> MDIRGRKMKKPPACVQCRKRKIGCDRVKPICGNCMKHNKMDCFYPDVPGQYVPSSSSSSNTRQVANGPYLNSYYASRRVSKETAALLQKNPELASLEQIREYNTRLQLLNAQNQLNNRSSAANATLNQQHTQYIPKSVPSLESKPVTSANESSTPLNWVQGPAIFHMLTSP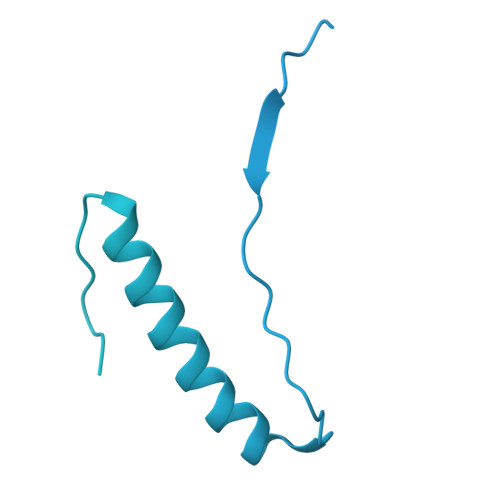YTQDEIINHEMNFLKGRLLELQEITGKKITGVNLDLKQDSSAQMQSSHSNRNQEEFLTIKKRKLSEDGVTDGDGKPIPESERRPHLNEFKDLDPQFLDTNKVFNVFNSAISEEGRNRLWLLPKNINKSSIFQIQYLIERDPFLFKFFNDLNILIETQFNGPLHDLVASRNSIERNSGISQILKFPSQSITQTLINKYLSTITETNSILPILKPKRLLPIVEQLFPSNTINKPNSKDFETIFQVFSVTNDQLLNLGFITLCLLILFESLNSTVLIPLRDDEHLQLFNVLFNYLPLLKSNLTTLRFEIEKRSMCNIETLRFISLWKYYQFVMDTSSSSSFVIDYDEDMHMACLLSLNHETQNQSHILTWNFIFKNYCWRHLFLGQLPLLMSEPFTNSTPIIDPLLNNDFELIDFEVNLMKYLQSKDQQLSIDKIIQLIKLLKNKNIEVSQGCLTTPSIINNIMDSLIYRNSMLYLNFYLLLQFETLKNYAKFNEILEDFLELSRETLFFVFSNLANIKFAGHEFTFINKSIVVLQTLVLMLLALYQRSFDSSKRTNDANEISEQTDIHSNNDNSKRIKNKNVIHLIINKIAMLLSDYSKNCKKQNKLIENLIIKIKTISKYIKNLEENKVTTSADSNYSINNGFSGISAEQLIKLNHELSKISESLIKTDFYEQRKNSTVSNGVLGAAAPVDSDANSDTFGLTKENFNEVFEAIRS> MGSHHHHHHSSGLVPRGSHMFKREEIIEMANKDFEKAWIETKDLIKAKKINESYPRIKPVFGKTHPVNDTIENLRQAYLRMGFEEYINPVIVDERDIYKQFGPEAMAVLDRCFYLAGLPRPDVGLSDEKISQIEKLGIKVSEHKESLQKILHGYKKGTLDGDDLVLEISNALEISSEMGLKILEDVFPEFKDLTAVSSKLTLRSHMTSGWFLTVSDLMNKKPLPFKLFSIDRCFRREQKEDKSHLMTYHSASCAIAGEGVDINDGKAIAEGLLSQFGFTNFKFIPDEKKSKYYTPETQTEVYAYHPKLKEWLEVATFGVYSPVALSKYGIDVPVMNLGLGVERLAMISGNFADVREMVYPQFYEHKLNDRNVASMVKLDKVPVMDEIYDLTKELIESCVKNKDLKSPCELAIEKTFSFGKTKKNVKINIFEKEEGKNLLGPSILNEIYVYDGNVIGIPESFDGVKEEFKDFLEKGKSEGVATGIRYIDALCFKITSKLEEAFVSNTTEFKVKVPIVRSLSDINLKIDDIALKQIMSKNKVIDVRGPVFLNVEVKIEXXXXXX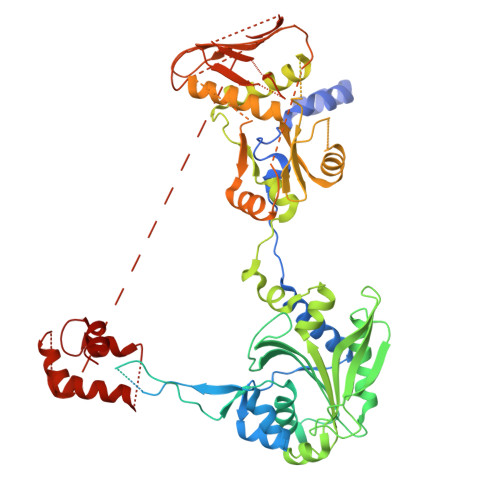XXXXXXXXXXXXXXXXXXXXXXXXXXXXXXXXXXXXXXXXXXXXXXXXXXXXXXXXXXXXXXXXXXXXXXXXXXXXXXXXXXXXXXXXXXXXXXXXXXXXXXX>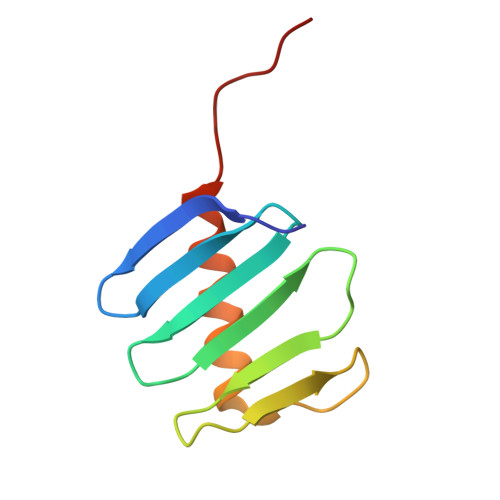 SAQLLKSVFVKNVGWATQLTSGAVWVQFNDGSQLVVQAGVSSISYTSPNGQTTRYGENEKLPDYIKQKLQCLSSILLMFSNPTPNFH5-benzyl-N-[(3S)-5-methyl-4-oxo-2,3,4,5-tetrahydro-1,5-benzoxazepin-3-yl]-1,2-oxazole-3-carboxamide | C21 H19 N3 O4 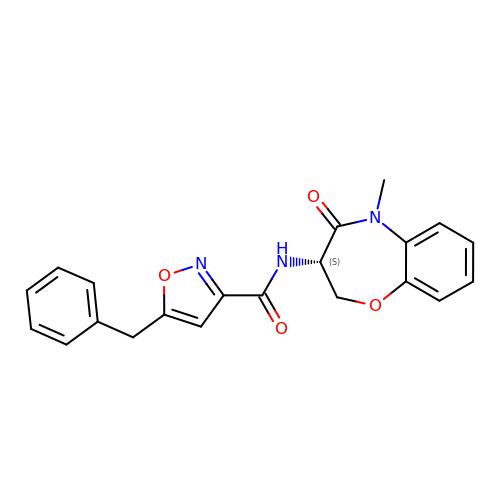| KNOUWGGQMADIBV-KRWDZBQOSA-N3-[[1-[(2~{S},3~{S})-1-methyl-6-oxidanylidene-2-phenyl-piperidin-3-yl]carbonyl-4-oxidanyl-piperidin-4-yl]methyl]quinazolin-4-one | C27 H30 N4 O4 | 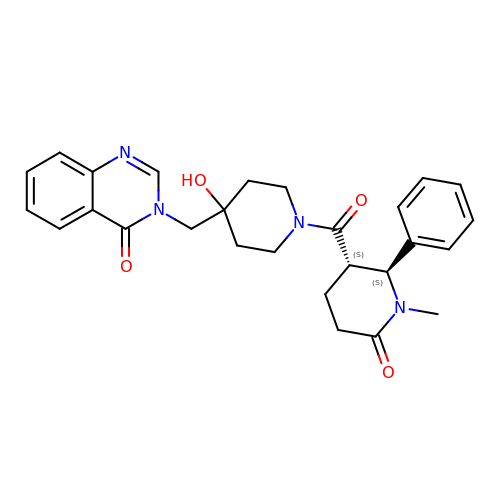LFWWCQUMVDUXSY-XUZZJYLKSA-N>[2x]MAPAEILNGKEISAQIRARLKNQVTQLKEQVPGFTPRLAILQVGNRDDSNLYINVKLKAAEEIGIKATHIKLPRTTTESEVMKYITSLNEDSTVHGFLVQLPLDSENSINTE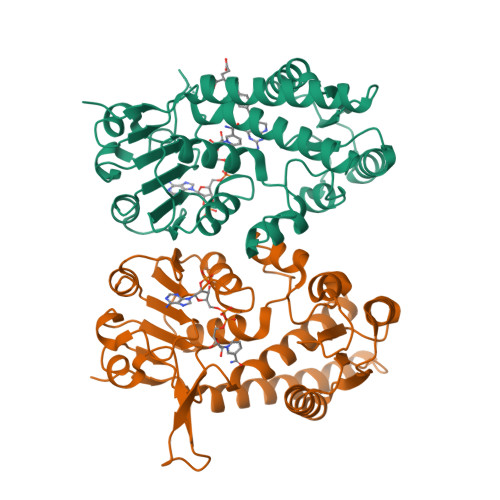EVINAIAPEKDVDGLTSINAGRLARGDLNDCFIPCTPKGCLELIKETGVPIAGRHAVVVGRSKIVGAPMHDLLLWNNATVTTCHSKTAHLDEEVNKGDILVVATGQPEMVKGEWIKPGAIVIDCGINYVPDDKKPNGRKVVGDVAYDEAKERASFITPVPGGVGPMTVAMLMQSTVESAKRFLEKFKPGKWMIQ> MGSDKIHHHHHHMIIGNCLILKDFSSEPFWGAVEIENGTIKRVLQGEVKVDLDLSGKLVMPALFNTH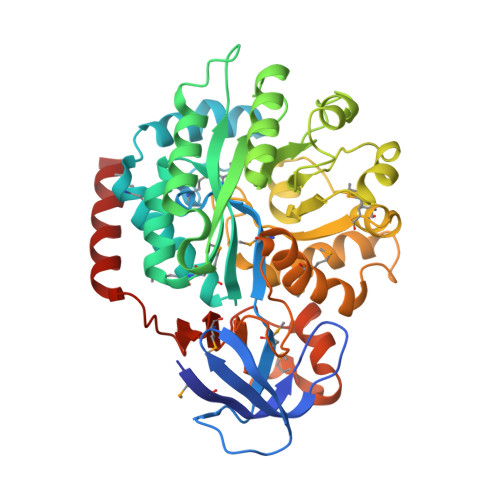THAPMTLLRGVAEDLSFEEWLFSKVLPIEDRLTEKMAYYGTILAQMEMARHGIAGFVDMYFHEEWIAKAVRDFGMRALLTRGLVDSNGDDGGRLEENLKLYNEWNGFEGRIFVGFGPHSPYLCSEEYLKRVFDTAKSLNAPVTIHLYETSKEEYDLEDILNIGLKEVKTIAAHCVHLPERYFGVLKDIPFFVSHNPASNLKLGNGIAPVQRMIEHGMKVTLGTDGAASNNSLNLFFEMRLASLLQKAQNPRNLDVNTCLKMVTYDGAQAMGFKSGKIEEGWNADLVVIDLDLPEMFPVQNIKNHLVHAFSGEVFATMVAGKWIYFDGEYPTIDSEEVKRELARIEKELYSS>[4x]MQRVTITLDDDLLETLDSLSQRRGYN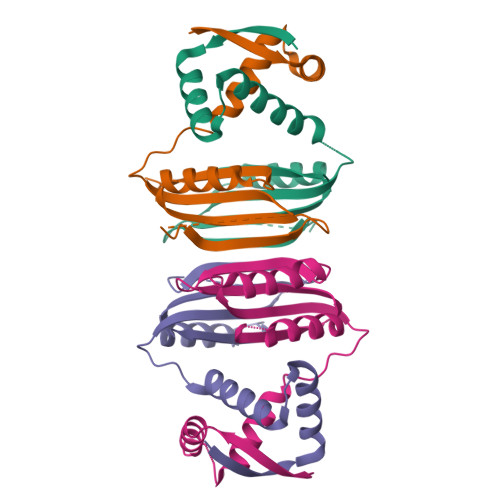NRSEAIRDILRSALAQEATQQHGTQGFAVLSYVYEHEKRDLASRIVSTQHHHHDLSVATLHVHINHDDCLEIAVLKGDMGDVQHFADDVIAQRGVRHGHLQCLPKED> GGPPQQVDQQETWRTNFYYNDVFTWSVADAPGSILYTVQHSPQNNPFTAVLSQMYAGWAGGMQFRFAVAGSGAFGGRVAAA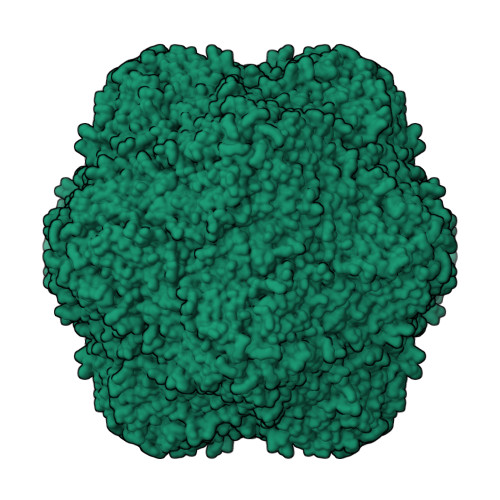VIPPGIEIGPGLEVRQFPHVVIDARSLEPVTNTMPDLRPNMYHPTGDPGLVPTLVLAVYNALINPFGGSTSAIQVTVETRPSEDFEFVMIRAP2-(5-{5-[AMINO(IMINIO)METHYL]-1H-BENZIMIDAZOL-2-YL}-2'-FLUORO-6-OXIDO-1,1'-BIPHENYL-3-YL)SUCCINATE | C24 H17 F N4 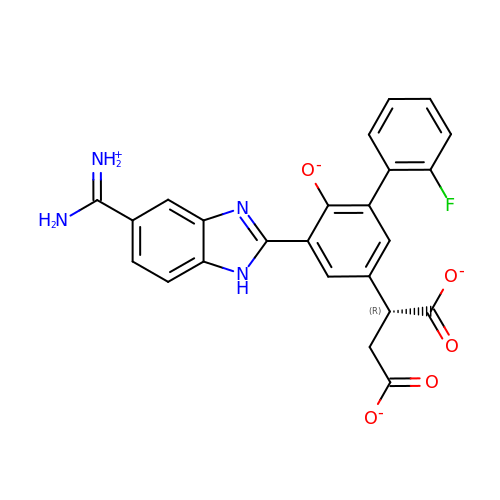O5 | XCOFROALSAFROV-CQSZACIVSA-L>[4x]MGERESKT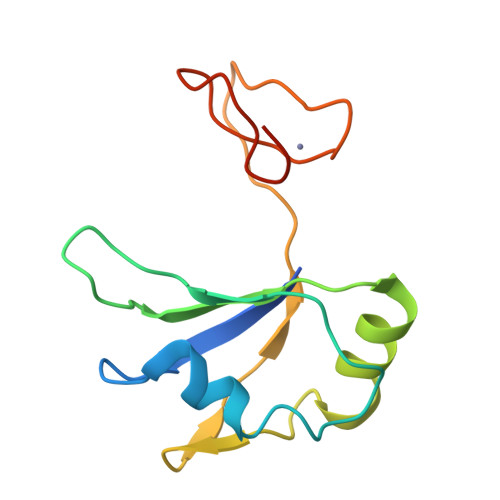IMLRGLPTTITESDIREMMESFEGPQPADVRLMKRKTGVSRGFAFVEFYHLQDATSWMEANQKKLVIQGKHIAMHYSNPRPKFEDWLCNKCGLNNFRKRLKCFRCGADKFD To date, several nucleoside transporters in mammals have been identified and classified into two SLC transporter families: concentrative nucleoside transporters (CNTs, the SLC28 family) and equilibrative nucleoside transporters (ENTs, the SLC29 family). Human CNT (hCNT) 3 (SLC28A3), one of the three members of the SLC28 family, is classified as a sodium–nucleoside or proton–nucleoside symporter. Compared with the other two members, hCNT3 has the broadest distribution, substrate specificity, and transport activity for nucleoside-derived drugs. hCNT3 is also an important mediator of drug response and resistance. Previous studies have shown that the truncated isoform (Δ1–69) of hCNT3, named CNT3ins, is an endoplasmic reticulum membrane protein with nucleoside transport activity.

Here, we report the cryo-EM structure of CNT3ins at an overall resolution of 3.6 Å. Then, we tried to purify CNT3ins in 0.1% (w/v) digitonin, which has also been used for the structural determination of human γ-secretase, and analyzed its structure using single-particle cryo-EM. The final three-dimensional (3D) density map was reconstructed from 99,489 particles with C3 symmetry, reaching an overall resolution of 3.6 Å. The processing scheme for structural determination is summarized in S5 Fig. CNT3ins consists of three protomers, a trimeric shamrock-shaped architecture that is formed through trimeric contacts of the central helices from each protomer. In the structure of CNT3ins, density is clearly resolved for residues 100–614 of each protomer, which can be divided into the core domain and additional N-terminal transmembrane helices (TMs). Each protomer of hCNT3 is formed by 11 TMs (TM1–11), which is consistent with the previously predicted 11 TM topology of hCNTs. The core domain of hCNT3 is composed of two subdomains, including the scaffold domain (TM4, TM5, TM6, TM9, and IH2) and the transport domain (IH3, HP1, TM7, TM8, IH4, HP2, TM10, and TM11). Considering that the structure of CNT3ins was obtained without nucleoside and no sodium ions were observed in the structure of CNT3ins, we used the structural superposition to identify the putative nucleoside and sodium binding sites of hCNT3. As superposition shows, the residues involved in nucleoside binding of hCNT3 (Q341, T342, E343, V375, F563, E519, N565, and S568) and vcCNT are identical, which indicates that hCNT3 possesses similar nucleoside selectivity to vcCNT. The observed position of the transport domain indicates an inward-facing state of hCNT3.

>[3x]MEDDDEEMQQKGCLERRYDTVCGFCRKHKTTLRHIIWGILLAGYLVMVISACVLNFHRALPLFVITVAAIFFVVWDHLMAKYEHRIDEMLSPGRRLLNSHWFWLKWVIWSSLVLAVIFWLAFDTAKLGQQQLVSFGGLIMYIVLLFLFSKYPTRVYWRPVLWGIGLQFLLGLLILRTDPGFIAFDWLGRQVQTFLEYTDAGASFVFGEKYKDHFFAFKVLPIVVFFSTVMSMLYYLGLMQWIIRKVGWIMLVTTGSSPIESVVASGNIFVGQTESPLLVRPYLPYITKSELHAIMTAGFSTIAGSVLGAYISFGVPSSHLLTASVMSAPASLAAAKLFWPETEKPKITLKNAMKMESGDSGNLLEAATQGASSSISLVANIAVNLIAFLALLSFMNSALSWFGNMFDYPQLSFELICSYIFMPFSFMMGVEWQDSFMVARLIGYKTFFNEFVAYEHLSKWIHLRKEGGPKFVNGVQQYISIRSEIIATYALCGFANIGSLGIVIGGLTSMAPSRKRDIASGAVRALIAGTVACFMTACIAGILSSTPVDINCHHVLENAFNSTFPGNTTKVIACCQSLLSSTVAKGPGEVIPGGNHSLYSLKGCCTLLNPSTFNCNGISNTFLEWSHPQFEK>GSHMTNTGGRKPDEGERYRAILETAARLICDRGYEGTSMQEIAAACRMTKAGLYHHIQNKEQLLFAIMNYGMDLFEEQVLSRVQDIANPVERLRACMRHNILLVTRGWSKEVIIILHEHATLTGETRAFIDARKKKYVDFLEEAFSQASQQGLI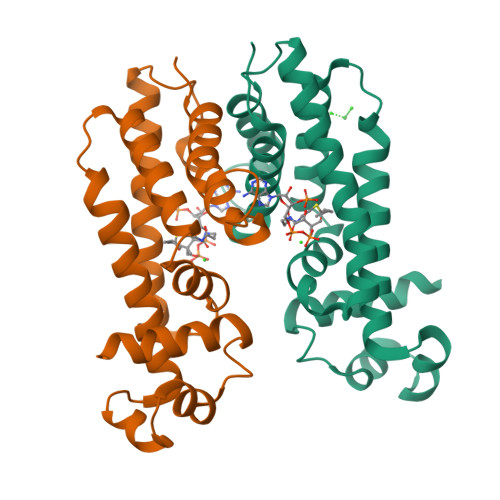RPVDPTVGAFSFLGMVLWIYKWFKPDGRLTDEQIADGMVGMLFPPFAAAGDTAGQAGPSPLRMVPSVSATGTDSEDA[2x]> GHTEIVKFLVQFGV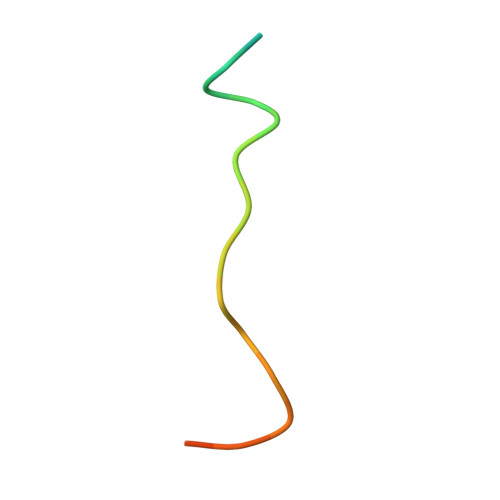NVNAADSDG>[3x]MTGSNRRANAGRKTQPKPQRKPRAPRRPKVQNAPRIQQGGGPVPLLESNSNMRQMHNGMTRVVGSDYLGVVSVAGNPADAAAKVRKVLSVSPSSFPGTRLTQMSDLWERYVFRQFRVRYVPSVPNTLACQVMVYQDTDPQDDPTAIKDADALLRQATAQTGSQQWNFNSAKVIHLAKRSDNQLYYTGPVKENPRFNQQGVVYFIQVSQALDMNGKP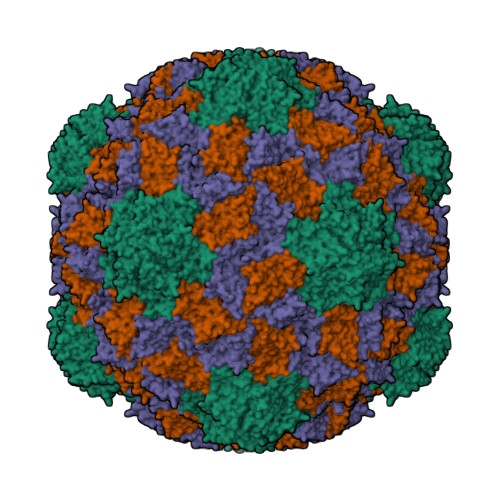LTADMECGSLYVDWVIDFQTPQVNPSAVEARLPSAGFFTRQILVNDKLTFAAQASLTVALTALSATPKVWLEGPTRVDLATLGGPGGNLVQIELTRAQPGDYTVKFVGCDSVTLVSSAPIA Even though constrained helical interaction motifs generally show a tendency to inhibit PPIs,1a only very few have been reported to directly target transcription factors with sufficient affinity to enable the inhibition of complex assembly.12a, 14 The nuclear transcription factor Y (NF‐Y)15 is a trimeric complex (NF‐YA/B/C) that binds to a particular DNA sequence (CCAAT box), thereby activating genes involved in regulation of the cell cycle and DNA repair. NF‐Y subunits B and C form a stable heterodimer, which by itself does not possess relevant affinity to DNA target sequences (CCAAT box DNA). Only upon availability and binding of the third subunit (NF‐YA) is the transcriptionally active trimeric complex formed and DNA binding occurs with affinity values in the low nanomolar range. In this study, we aimed to inhibit the interaction between the NF‐YB/C heterodimer (light/dark grey) and NF‐YA (green) to prevent transcription‐factor assembly and DNA (blue) binding.

Within the NF‐YA helix, we identified five solvent‐exposed amino acids (Y272, H273, L276, Q280, A283), which were used for crosslink incorporation. This resulted in four stapled helices, two with i,i+7 (macrocycle A and C) and two with i,i+4 (macrocycle B and D) crosslinks, all of which were introduced in two different lengths of the binding motif (16‐mer 5 and 19‐mer 2). ITC measurements also confirm the expected 1:1 binding stoichiometry for peptide and NF‐YB/C. To investigate the binding mode, we co‐crystalized 2‐C in complex with NF‐YB/C, which provided crystals that diffract to 1.8 Å (space group P212121). Superimposition of 2‐C and corresponding residues in PBM shows a good overlap, thus confirming an analogous binding mode (RMSD=0.59 Å). The overlay of 2‐DN, 2‐C, and PBM in their bound state indicates an almost identical peptide conformation. Linear peptide 2 shows a very small helical content (13 %, green), while i,i+7 stapled peptide 2‐C exhibits high α‐helicity (81 %, blue). Compared to peptide 2, both peptides with a fully α‐methylated macrocycle (2‐C and 2‐D) exhibit a reduced entropic penalty while the contributions by binding enthalpy are decreasing. Presumably, the bioactive conformation of the peptide observed in the crystal structures of PBM, 2‐C, and 2‐DN is perturbed by an α‐methyl group at position 272.

> XVNAKQYXRILKRRXARAKLX;> GPSFREQDIYLPIANVARIMKNAIPQTGKIAKDAKECVQECVSEFISFITSEASERCHQEKRKTINGEDILFAMSTLGFDSYVEPLKLYLQKFRE;> GPMEEIRNLTVKDFRVQELPLARIKKIMKLDEDVKMISAEAPVLFAKAAQIFITELTLRAWIHTEDNKRRTLQRNDIAMAITKFDQFDFLIDIVPR4-(thiophen-3-yl)benzoic acid | C11 H8 O2 S | 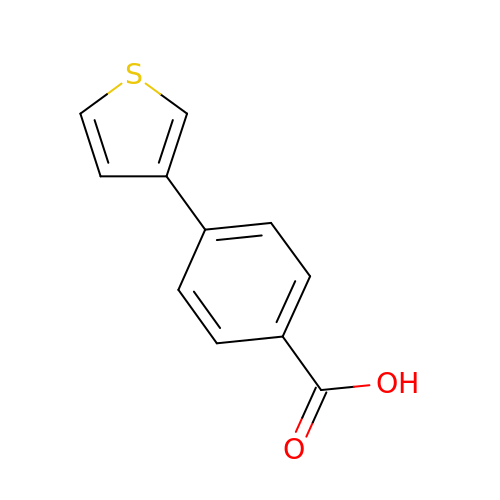FISAUHGRILVMDP-UHFFFAOYSA-N>MEKKTIVLGVIGSDCHAVGNKILDHAFTNAGFNVVNIGVLSPQELFIKAAIETKADAILVSSLYGQGEIDCKGLRQKCDEAGLEGILLYVGGNIVVGKQHWPDVEKRFKDMGYDRVYAPGTPPEVGIADLKKDLNIE[2x];>MELKNKKWTDEEFHKQREEVLQQWPTGKEVDLQEAVDYLKKIPAEKNFAEKLVLAKKKGITMAQPRAGVALLDEHIELLRYLQDEGGADFLPSTIDAYTRQNRYDECENGIKESEKAGRSLLNGFPGVNFGVKGCRKVLEAVNLPLQARHGTPDSRLLAEIIHAGGWTSNEGGGISYNVPYAKNVTIEKSLLDWQYCDRLVGFYEEQGVHINREPFGPLTGTLVPPSMSNAVGITEALLAAEQGVKNITVGYGECGNMIQDIAALRCLEEQTNEYLKAYGYNDVFVTTVFHQWMGGFPQDESKAFGVIVTATTIAALAGATKVIVKTPHEAIGIPTKEANAAGIKATKMALNMLEGQRMPMSKELETEMAVIKAETKCILDK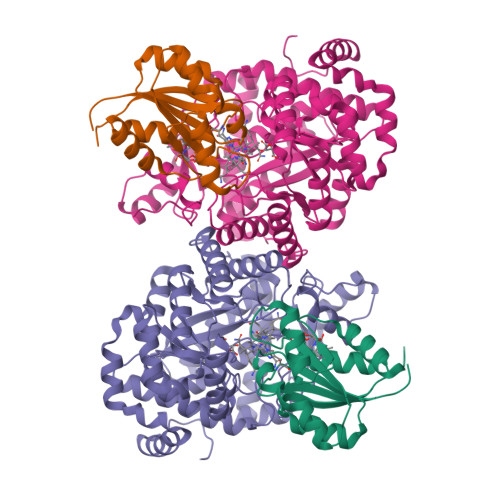MFELGKGDLAIGTVKAFETGVMDIPFGPSKYNAGKMMPVRDNLGCVRYLEFGNVPFTEEIKNYNRERLQERAKFEGRDVSFQMVIDDIFAVGKGRLIGRPE[2x]>MPYIEKLELKGFKSYGNKKVVIPFSKGFTAIVGANGSGKSNIGDAILFVLGGLSAKAMRASRISDLIFAGSKNEPPAKYAEVAIYFNNEDRGFPIDEDEVVIRRRVYPDGRSSYWLNGRRATRSEILDILTAAMISPDGYNIVLQGDITKFIKMSPLERRLLIDDISGIAEYDSKKEKALEE[2x];>MEKEKKNVFMRTFEAISRNFSEIFAKLSPGGSARLILENPEDPFSGGLEIEAKPAGKDVKRIEAMSGGEKALTALAFVFAIQKFKPAPFYLFDEIDAHLDDANVKRVADL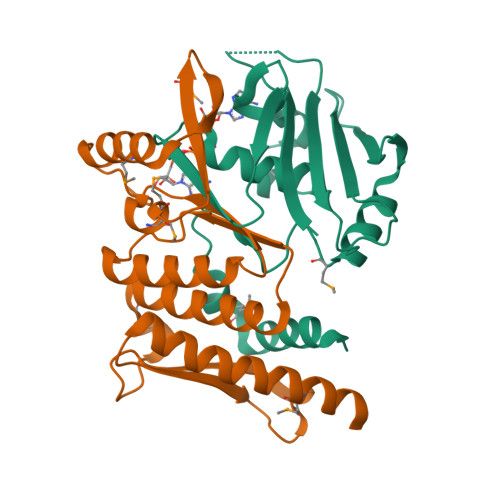IKESSKESQFIVITLRDVMMANADKIIGVSMRDGVSKVVSLSLEKAMKILEEIRKKQGWEHGN[2x]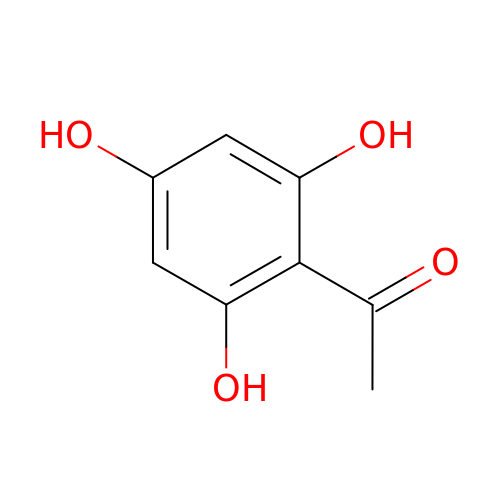1-[2,4,6-tris(oxidanyl)phenyl]ethanone | C8 H8 O4 | XLEYFDVVXLMULC-UHFFFAOYSA-N CTP synthase (CTPS) catalyzes the final, rate-limiting step of de novo CTP biosynthesis (Lieberman, 1956). Each CTPS monomer consists of a glutaminase domain and an amido-ligase domain connected by an alpha helical linker. Glutamine hydrolysis in the glutaminase domain produces ammonia which is transferred through a channel into the amido-ligase domain, where it is ligated to UTP to form CTP in an ATP-dependent process. Budding yeast have two CTPS isoforms, Ura7 and Ura8, which share 78 % identical residues.

To test whether CTPS filament assembly has a direct effect on enzyme activity, we generated mutations at H360 in the assembly interface of Ura7 that either disrupted or stabilized filaments. To mimic protonation at H360, we mutated it to arginine, with the expectation that a constitutive positive charge might support polymerization at neutral pH. Indeed, we found that Ura7-H360R robustly assembles filaments at pH 7.4 which, like the wild-type protein, assemble only in the presence of substrate or product ligands. To confirm that H360R does not alter filament structure, we determined a 6.7 Å cryo-EM structure of substrate-bound Ura7, which is indistinguishable from wildtype at this resolution. Thus, reversible assembly of H360R into wiltype-like filaments is pH-insensitive. At pH 7.4 Ura7-H360A is completely tetrameric and had the highest activity, wild-type enzyme has a background of single filaments and had slightly lower activity, and Ura7-H360R had robust filament assembly and the lowest observed activity. This suggests that filament assembly in itself acts as an allosteric inhibitor of enzyme activity, with kcat reduced likely as a consequence of the constricted ammonia channel we observe in the filament structure. Based on our in vitro findings, we predicted that the pH-insensitive Ura7-H360R would constitutively assemble polymers in cells. But surprisingly, its localization was very similar to wildtype, diffuse during log phase growth and assembled into foci upon nutritional deprivation. However, Ura7-H360R-GFP assembly and disassembly kinetics are dysregulated.

>MKYVVVSGGVISGIGKGVLASSTGMLMKTLGLKVTSIKIDPYMNIDAGTMSPLEHGECFVLDDGGETDLDLGNYERYLGVTLTKDHNITTGKIYSHVIAKERKGDYLGKTVQIVPHLTNAIQDWIERVAKIPVDDTGMEPDVCIIELGGTVGDIESAPFVEALRQFQFKVGKENFALIHVSLVPVIHGEQKTKPTQAAIKGLRSLGLVPDMIACRCSETLDKPTIDKIAMFCHVGPEQVVNVHDVNSTYHVPLLLLEQKMIDYLHARLKLDEISLTEEEELLSKWKATTGNFDETVKIALVGKYTNLKDSYLSVIKALEHSSMKCRRKLDIKWVEATDLEPEAQESNKTKFREAWNMVSTADGILIPGGFGVRGTEGMVLAARWARENHIPFLGVCLGLQIATIEFTRSVLGRKDSHSAEFYPDIDEKNHVVVFMMRLGLRPTFFQNETEWSQIKKLYGDVSEVHERHRHRYEINPKMVDELENNGLIFVGKDDTGKRCEILELKNHPYYIATQYHPEYTSKVLDPSKPFLGLVAASAGILQDVIEGKYDLEA[8x]> LSITTPEQRIEKAKGETAYLPCKFTLSPEDQGPLDIEWLISP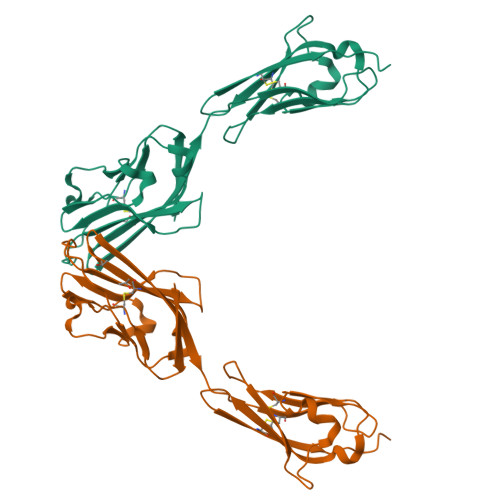SDNQIVDQVIILYSGDKIYDNYYPDLKGRVHFTSNDVKSGDASINVTNLQLSDIGTYQCKVKKAPGVANKKFLLTVLVKPSGTRCFVDGSEEIGNDFKLKCEPKEGSLPLQFEWQKLSDSQTMPTPWLAEMTSPVISVKNASSEYSGTYSCTVQNRVGSDQCMLRLDVVPPS> MEDNYAADVQRQFNRTAFDSLYKICYNSLVQKNGSTIDFQKQIDCHQRLI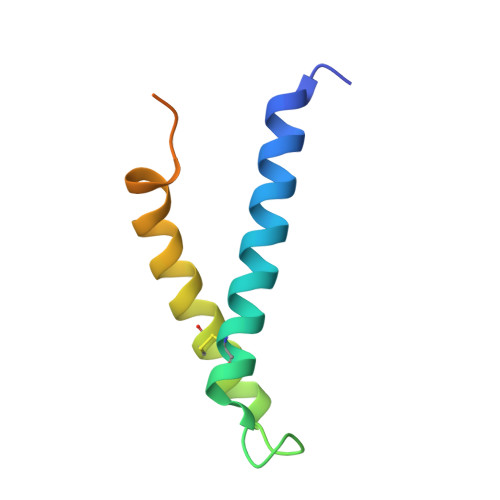QVFAKIAPIVVKVEQDAASSGGAAAGGEDEE> HMNAEINPLHAYFKLPNTV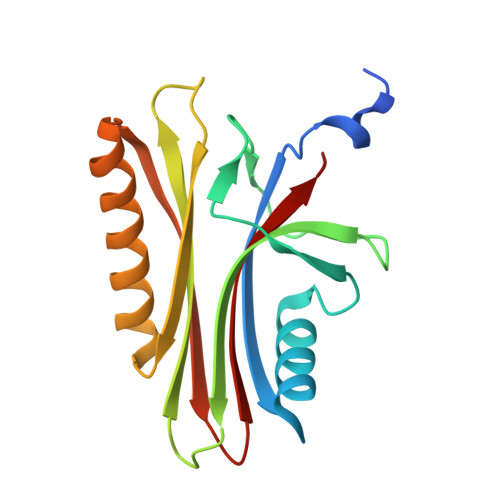SLVAGSSEGETPLNAFDGALLNAGIGNVALIRISSIMPPEAEIVPLPKLPMGALVPTAYGYIISDVPGETISAAISVAIPKDKSLCGLIMEYEGKCSKKEAEKTVREMAKIGFEMRGWELDRIESIAVEHTVEKLGCAFAAAALWYK2-({6-{3-[AMINO(IMINO)METHYL]PHENOXY}-3,5-DIFLUORO-4-[(1-METHYL-3-PHENYLPROPYL)AMINO]-2-PYRIDINYL}OXY)BENZOIC ACID | C29 H26 F2 N4 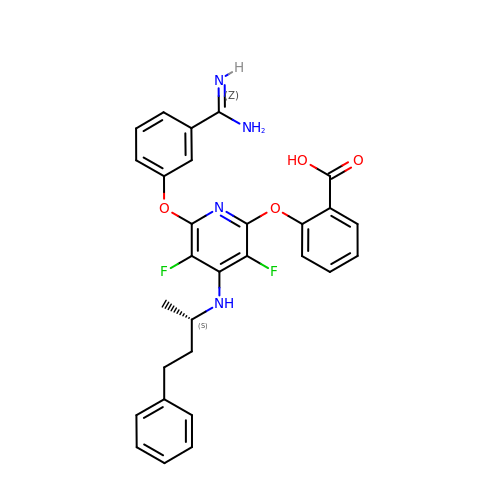O4 | BUZNVJZUYOBGFM-KRWDZBQOSA-N>[16x]MDFETGEHQYQYKDILSVFEDAFVDNFDCKDVQDMPKSILSKEEIDHIIMSKDAVSGTLRLFWTLLSKQEEMVQKFVEEVLRINYKFLMSPIKTEQRQPSMMTRMYIEQRDRLYNDNQVFAKYNVSRLQPYLKLRQALLELRPAKNVLIDGVLGSGKTWVALDVCLSYKVQCKMDFKIFWLNLKNCNSPETVLEMLQKLLYQIDPNWTSRSDHSSNIKLRIHSIQAELRRLLKSKPYENCLLVLLNVQNAKAWNAFNLSCKILLTTRFKQVTDFLSAATTTHISLDHHSMTLTPDEVKSLLLKYLDCRPQDLPREVLTTNPRRLSIIAESIRDGLATWDNWKHVNCDKLTTIIESSLNVLEPAEYRKMFDRLSVFPPSAHIPTILLSLIWFDVIKSDVMVVVNKLHKYSLVEKQPKESTISIPSIYLELKVKLENEYALHRSIVDHYNIPKTFDSDDLIPPYLDQYFYSHIGHHLKNIEHPERMTLFRMVFLDFRFLEQKIRHDSTAWNAS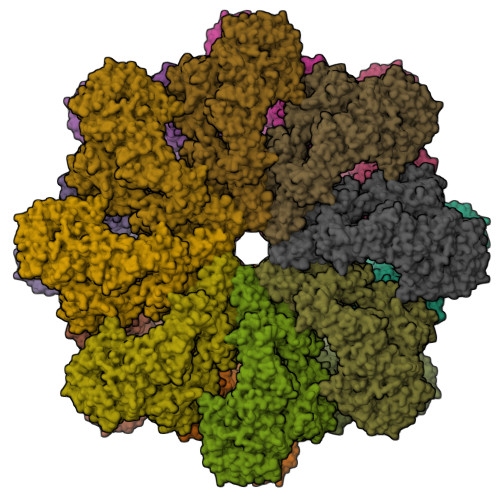GSILNTLQQLKFYKPYICDNDPKYERLVNAILDFLPKIEENLICSKYTDLLRIALMAEDEAIFEEAHKQVQRFDDRVWFTNHGRFHQHRQIINLGDNEGRHAVYLHNDFCLIALASGQILLTDVSLEGEDTYLLRDESDSSDILRMAVFNQQKHLITLHCNGSVKLWSLWPDCPGRRHSGGSKQQLVNSVVKRFIGSYANLKIVAFYLNEDAGLPEANIQLHVAFINGDVSILNWDEQDQEFKLSHVPVLKTMQSGIRCFVQVLKRYYVVCTSNCTLTVWDLTNGSSNTLELHVFNVENDTPLALDVFDERSKTATVLLIFKYSVWRLNFLPGLSVSLQSEAVQLPEGSFITCGKRSTDGRYLLLGTSEGLIVYDLKISDPVLRSNVSEHIECVDIYELFDPVYKYIVLCGAKGKQVVHVHTLRSVSGSNSHQNREIAWVHSADEISVMTKACLEPNVYLRSLMDMTRERTQLLAVDSKERIHLIKPAISRISEWSTITPTHAASNCKINAISAFNDEQIFVGYVDGVIIDVIHDTALPQQFIEEPIDYLKQVSPNILVASAHSAQKTVIFQLEKIDPLQPNDQWPLMMDVSTKYASLQEGQYIILFSDHGVCHLDIANPSAFVKPKDSEEYIVGFDLKNSLLFLAYENNIIDVFRLIFSCNQLRYEQICEEEIAQKAKISYLVATDDGTMLAMGFENGTLELFAVENRKVQLIYSIEEVHEHCIRQLLFSPCKLLLISCAEQLCFWNVTHMRNNQLEREQKRRRSRRHKQHSVTQEDAVDAAPIAADIDVDVTFVADEFHPVNRGTAELWRNKRGNAIRPELLACVKFVGNEARQFFTDAHFSHFYAIDDEGVYYHLQLLELSRLQPPPDPVTLDIANQYEDLKNLRILDSPLMQDSDSEGADVVGNLVLEKNGGVARATPILEEASS>[2x]AESTLGAAAAQSGRYFGTAIASGRLSDSTYTSIAGREFNMVTAENEMKIDATEPQRGQFNFSSADRVYNWAVQNGKQVRGHTLAWHSQQPGWMQSLSGSALRQAMIDHINGVMAHYKGKIVQWDVVNEAFADGSSGARRDSNLQRSGNDWIEVAFRTARAADPSAKLCYNDYNVENWTWAKTQA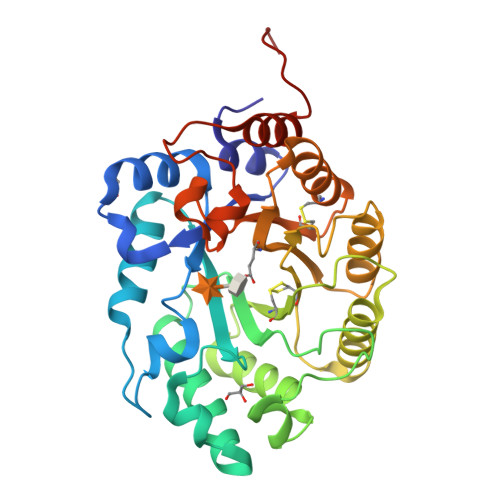MYNMVRDFKQRGVPIDCVGFQSHFNSGSPYNSNFRTTLQNFAALGVDVAITELDIQGAPASTYANVTNDCLAVSRCLGITVWGVRDSDSWRSEQTPLLFNNDGSKKAAYTAVLDALNGGDSSEPPADGG>[12x]MSSTPSNQNIIPIIKKESIVSLFEKGIRQDGRKLTDYRPLSITLDYAKKADGSALVKLGTTMVLAGTKLEIDKPYEDTPNQGNLIV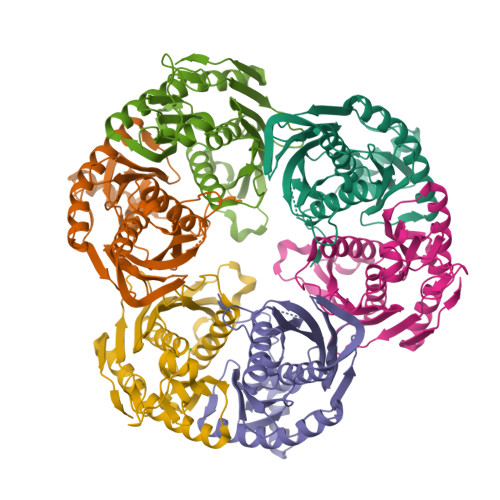NVELLPLAYETFEPGPPDENAIELARVVDRSLRDSKALDLTKLVIEPGKSVWTVWLDVYVLDYGGNVLDACTLASVAALYNTKVYKVEQHSNGISVNKNEVVGKLPLNYPVVTISVAKVDKYLVVDPDLDEESIMDAKISFSYTPDLKIVGIQKSGKGSMSLQDIDQAENTARSTAVKLLEELKKHLGI;>MREMLQVERPKLILDDGKRTDGRKPDELRSIKIELGVLKNADGSAIFEMGNTKAIAAVYGPKEMHPRHLSLPDRAVLRVRYHMTPFSTDERKNPAPSRREIELSKVIREALESAVLVELFPRTAIDVFTEILQADAGSRLVSLMAASLALADAGIPMRDLIAGVAVGKADGVIILDLNETEDMWGEADMPIAMMPSLNQVTLFQLNGSMTPDEFRQAFDLAVKGINIIYNLEREALKSKYVEFKEEGV[12x]> APVPVT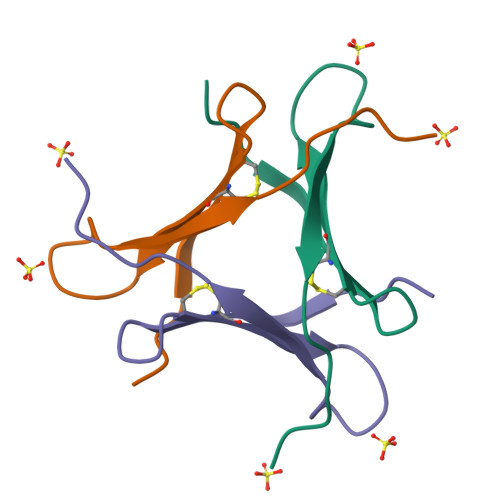KLVCDGDTYKCTAYLDFGDGRWVAQWDTNVFHTG> MGHHHHHHHHHHSSGHIEGRHMKRIAIVGAGQSGLQLGLGLLAAG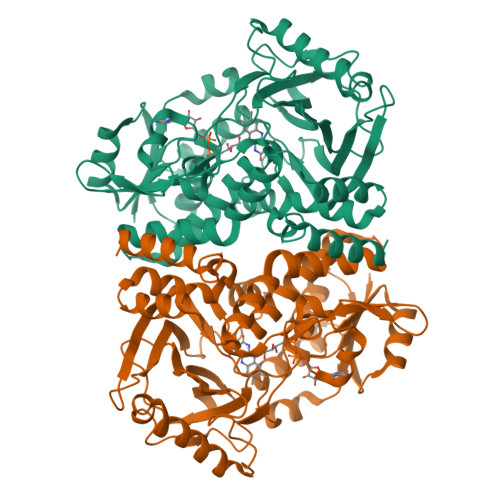YEVTMFSNRTGEDIRRGKVMSSQCMFDTSLQIERDLGLDHWASDCPTVDGIGLAVPHPEQKGAKVIDWAARLNASAQSVDQRLKIPAWMDEFQKKGGELVFKDAGIDELEACTQSHDLTLVASGKGEISKLFERDAHKSPYDKPQRALALTYVKGMAPREPFSAVCFNLIPGVGEYFVFPALTTTGPCEIMVFEGVPGGPMDCWADVKTPEEHLARSKWILDTFTPWEAERCKDIELTDDNGILAGRFAPTVRKPVATLPSGRKVLGLADVVVLNDPITGQGSNNAAKCADTYLKSILARGDGAADAAWMQQTFDRYWFGYAQWVTQWTNMLLAPPPPHVLNLLGSAGAVPPLASAFANGFDDPRTFFPWFADAAESERYIATCAAVA> MSVHIEAKQGEIAESILLPGDPLRAKYIAETFLEDVTCYNNVRGMLGFTGTYKGKRVSVQGTGMGVPSISIYVNELIQSYGVKNLIRVGTCGAIQKDVKVRDVIIAMTACTDSNMNRLTFPGFDFAPAA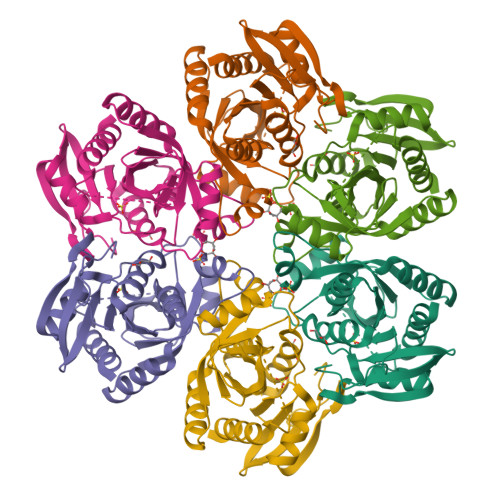NFDLLKKAYDAGTEKGLHVRVGNVLTADVFYRESMDMVKKLGDYGVLAVEMETTALYTLAAKYGVNALSVLTVSDHIFTGEETTSEERQTTFNEMIEIALDAAIQQ Sarcosine oxidase from Bacillus sp. (SoxB) recognizes the cyclic imino acids l‐proline (l‐Pro), d‐proline (d‐Pro), and l‐thioproline (l‐Tpr) as minor substrates.

The Tyr254Ala and Tyr254Gly mutants exhibited enhanced reactivity toward cyclic imino acids by eliminating this spatial interference. Crystallographic analysis of the mutants revealed an enlarged active site, which facilitated reactions with five‐membered cyclic imino acids. These mutations disrupted the electron delocalization associated with l‐Tpr, thereby eliminating charge transfer and substrate inhibition.

>[2x]STHFDVIVVGAGSMGMAAGYQLAKQGVKTLLVDAFDPPHTNGSHHGDTRIIRHAYGEGREYVPLALRSQELWYELEKETHHKIFTKTGVLVFGPKGESAFVAETMEAAKEHSLTVDLLEGDEINKRWPGITVPENYNAIFEPNSGVLFSENCIRAYRELAEARGAKVLTHTRVEDFDISPDSVKIETANGSYTADKLIVSMGAWNSKLLSKLNLDIPLQPYRQVVGFFESDESKYSNDIDFPGFMVEVPNGIYAGFPSFGGCGLKLGYHTFGQKIDPDTINREFGVYPEDESNLRAFLEEYMPGANGELKRGAVCMYTKTLDEHFIIDLHPEHSNVVIAAGFSGHGFKFSSGVGEVLSQLALTGKTEHDISIFSINRPALKESLQKTTIGSHHHHHH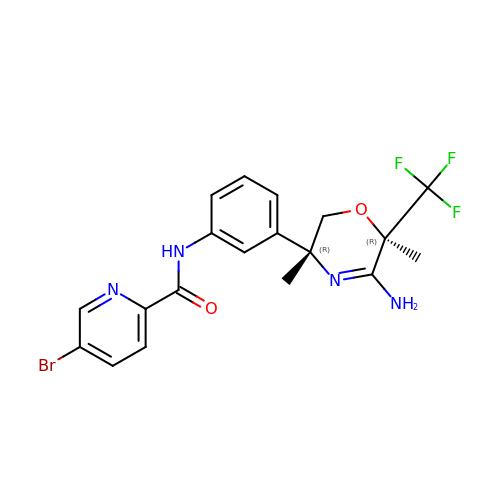~{N}-[3-[(3~{R},6~{R})-5-azanyl-3,6-dimethyl-6-(trifluoromethyl)-2~{H}-1,4-oxazin-3-yl]phenyl]-5-bromanyl-pyridine-2-carboxamide | C19 H18 Br F3 N4 O2 | YGNDEESWZOXXLA-ZWKOTPCHSA-N> SNARPAIRKRLLK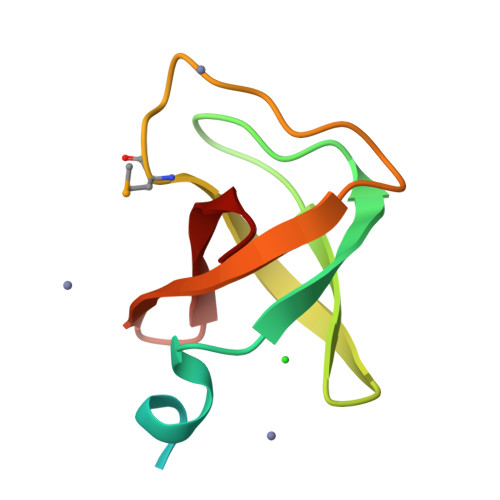PKVLDSSPRALVGHRAEVLEDVGATSGQVRLDGSIWSARSMDPTHTFAEGEIVSVIDIQGTTAIVWKEA>[2x]MGL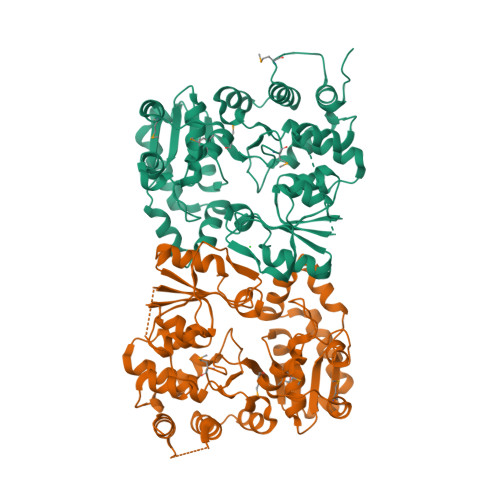AVFLPPYPFRGLKAPYLWMFYKYLHCATDSILFITGEDYLSVTDDEAQRARWEFDPASMASLGYELPNAQSMACHEYLTLDNAFYETLLSRHHHDPIKSFSAFLTERIPDLETELHALLDSKKGIIDQIDTFISICNCPSLEHVARTLGKEVMHIEIGPLRAPMYRNTAYLDFAGVNGGTEASARYEKCQAEFDIKASLGDLHNYFLEVLPPAEAATHSAAGVVLQVEDDSNLIAYNHDFTNISLLSYVRQRYEKEDILVRAHPGSLFRLRDDVFTIDDSANSLAFINQCNEVFTINSSVGLEAILTGKKTTVLGDCSYAFINELAGASATVNAAAFYLFSYLVPFDLVFNQEYLKFRLGHPEEREIVGKHIEFYSADMPGSLSQAAHSLSSLINEAISLEHHHHHH> MKKEFAVIGLGRFGGSICKALSEEGVEVMAMDIDEDKVNEYAKIASHAVIGDSTDESVLKNLGLRNFDHVIVAIGENIQASILT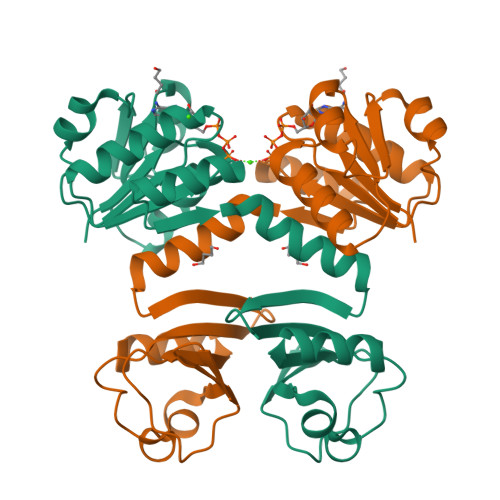TLILKELGVHTITVKAQNDYHEKVLSKIGADHIVHPERDMAKRIAHNIVSNNVLDYLELSEEHSLVEIVANSRLAGNTLLDLDIRAKYGINIVAIKRGKEVIVSPLATEVIHQEDILIVIGSVTDISRFEKRVLHTK Poly(ADP-ribose)glycohydrolase (PARG) and (ADP-ribosyl)hydrolase 3 (ARH3) are the main hydrolases of serine PAR- and MARylation, respectively, thus playing a pivotal role in signal silencing following DNA damage. ARH3 is the only known enzyme to reverse serine MARylation and is consequently responsible for the regulation of hundreds of ADP-ribosylated proteins following DNA damage. In contrast to PARG, the active site of ARH3 contains a catalytic binuclear magnesium centre. To understand the impact of the ARH3:substrate interaction on reaction efficiency, we crystallised ARH3 in complex with the chemically synthesised substrates: histone H2B peptide (aa 1–11) MARylated on Ser7 (H2BS7mar), dimeric ADP-ribose (dimer) and α-NAD+.

Furthermore, we solved the structure of wt Latimeria chalumnae ARH3 (LchARH3) in complex with meADPr. Interestingly, while we observe an open conformation in the H2BS7mar- and α-NAD+-bound structures, both the hARH3:dimer and LchARH3:meADPr complexes adopt a closed conformation. H2BS7mar and meADPr act similarly to chelants via the 1″ and 2″ oxygens. The interactions with either H2BS7mar or meADPr increase the Thr317-MgII distance by 0.9–1.6 Å relative to the ADPr-bound state, which breaks the coordinating bond and leads to an unusual five-coordinated distorted square-pyramidal geometry around the Mg2+ ion. The importance of this step can be observed in our LchARH:meADPr structure in which the ligand engages with the magnesium centre, but fails to displace Glu33 (Glu41 in hARH3) from MgII. Therefore, meADPr can act as an inhibitor of ARH3 instead of being hydrolysed. To assess whether the 1″-O-methyl moiety of ADPra1:n had an influence on the reaction, we performed inhibitor studies utilising free meADPr. Our results indicate that the latter acts as an inhibitor of the ARH3 reaction with comparable potency to ADPr.

>[2x]GPMVSLAQVRGALCGALLGDCMGAEFEGSDAVELPDVLEFVRLLEKEKKAGTLFYTDDTAMTRAVIQSLIAKPDFDEVDMAKRFAEEYKKEPTRGYGAGVVQVFKKLLSPKYSDVFQPAREQFDGKGSYGNGGAMRVASIALAYPNIQDVIKFARRSAQLTHASPLGYNGAILQALAVHFALQGELKRDTFLEQLIGEMERIEGGEMSASDAGEHDRPNEVKLPFCSRLKKIKEFLASSNVPKADIVDELGHGIAALESVPTAIYSFLHCMESDPDIPDLYNNLQRTIIYSISLGGDTDTIATMAGAIAGAYYGMDQVTPSWKRSCEAIVETEESAVKLYELYCKQLKTP6-[5-[6-(4-oxidanylcyclohexyl)oxy-1~{H}-pyrrolo[2,3-b]pyridin-5-yl]-1,2-oxazol-3-yl]pyridine-2-carboxamide 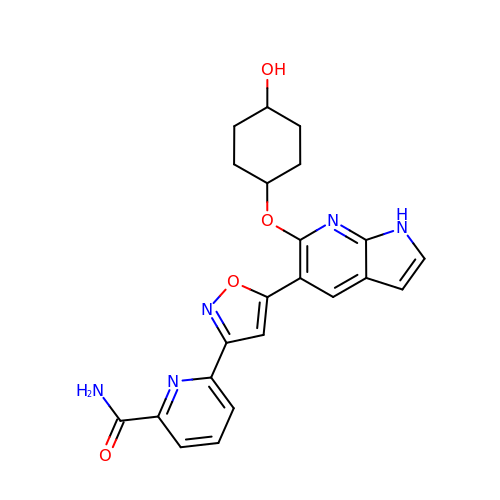| C22 H21 N5 O4 | HLYKWNVFHAYDMI-UHFFFAOYSA-N> GSHMKIYIQPLSVNSHTVEVLANSLPKIFNAEVFVLPASDVSLKCYNASRRQYNSTCILRMLPPIKVTLGVTGKDIYAKGMNFVFGEAELGGARAVLSVFRLTTADSELYRERVVKEAVHEIGHVLGLKHCSNNCVMRFSNSVQDVDRKPVSFCRECASKIRY

Archaemetzincins are metalloproteases occurring in archaea and some mammalia. They are distinct from all the other metzincins by their extended active site consensus sequence HEXXHXXGXXHCX4CXMX17CXXC featuring four conserved cysteine residues. The overall structure of AfAmzA resembles those of other metzincins, consisting of an upper N-terminal domain (NTD) and a lower helical C-terminal domain (CTD) with respect to the active site helix α2, which harbors two of the three zinc-binding histidines (H117EIGH121) and the catalytic base Glu118. On the other hand, as the homologous archaemetzincins from Methanopyrus kandleri (MkAmzA) and Methanocorpusculum labreanum (MlAmzA), AfAmzA exhibits a second zinc-binding site located in the CTD immediately below the catalytic zinc binding site and close to the eponymous, structurally important Met-turn.

The 6xHis-tag was removed by thrombin yielding the full-length protein with three additional residues preceding the start methionine (referred to as NHis-AfAmzA.). The first three amino acids of the NHis-AfAmzA construct employed in this study are the remainder of the N-terminal 6xHis-tag after thrombin cleavage and will be denoted by negative residue numbers, thus as Gly-3, Ser-2 and His-1. By the bidentate coordination of the (deprotonated) amino terminus and the carbonyl oxygen of Gly-3* the zinc-bound water is displaced from its spatial position between the zinc ion and the catalytic base. Furthermore, the metal-ligand interactions are similar to those observed in crystal structures of metzincins complexed with cognate proteinaceous inhibitors such as serralysins or MMPs. Contrary to substrates, the artificial N-terminal overhang is positioned in a parallel manner to the edge strand ß4 and does not form backbone-backbone interactions with this substrate-fixing element. The crystal structures of NHis-AfAmzA and nat-AfAmzA show rather large differences in the substrate-binding site. Despite different space groups and solvent contents, the conformations of the molecules in the new crystal forms are very similar to each other but at the same time they are substantially different from the original tetragonal form (NHis-AfAmzA) with respect to their active-site binding clefts.> MPAGGRLMKNLYHYHQYEITLESAVDSCKNHLQAAIGLLYSPQKCELVKLDNSGKLVDSYNRLKFNNLGVFEARFFNLNCELRWVNESNGNGTAVLLSESDITLTGFEKGLQEFITAIDQQYLLWGEPAKHPPNADGWQRLAEARIGKLDIPLDNPLKPKDRVFLTSEE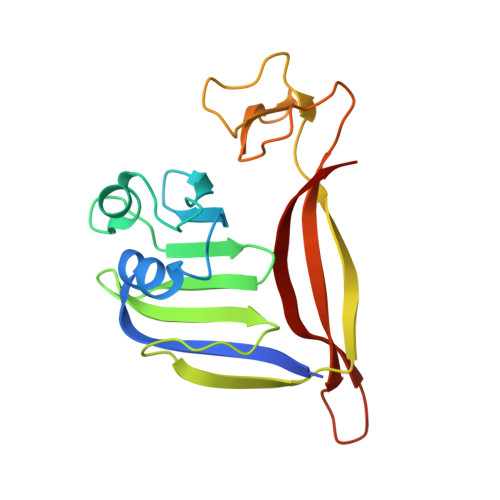YIAEVDDFGNCAVIDERLIKLEVK> MGSSHHHHHHSSGLVPRGSHMTTTISADQ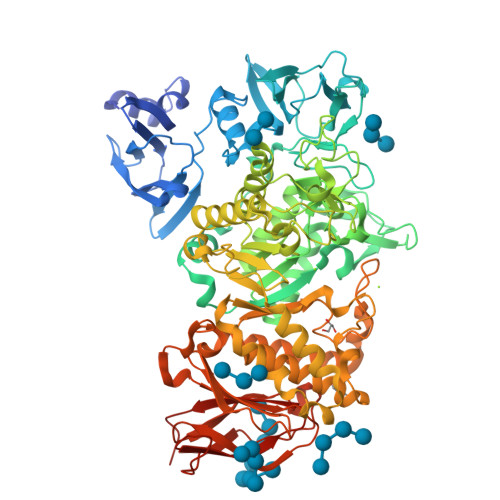VNQIIYNLHHDPFEILGCHLLEEGKNTKKWVVRAYLPKAEAAWVIRPTERKEDPMNSVHHPNFFECIIETPELNHYQLKVKEGEHEKVIYDPYAFSSPYLTDEDIYLFSEGNHHRIYEKLGAHVGEINGVKGVYFAVWAPNARNVSVIGDFNNWDGREHQMRKRNYTIWELFVPEIGSGTVYKYEIKNSEGHIYEKSDPYGFYREVRPNTASIVVDIDNIYQWHDEEWLEKRRNSDPLKQPVSVYEVHLGSWLHGSSAEKMPLLNGEADPVIVSEWNPGARFLSYYELAEKLIPYVKDMGYTHIELLPIAEHPFDGSWGYQVTGFYSPTSRFGRPEDFMYFVDKCHENGIGVILDWVPGHFPKDSHGLAYFDGTHLYEHADPRIGEHKEWGTLVFNYGRHEVRNFLVANVLFWFDKYHVDGIRVDAVASMLYRNYLRKEGEWIANEYGGDEHIEAVSFIREVNTLLFEYFPGILSIAEESTEWEKVSRPVAAGGLGFNLKWDMGWMHDMLDYFNIDPYFRQYHQNNVTFSMLYYYNENFMLALSHDEIVHGKSNMLGKMPGDEWQKYANVRALFTYMYTHPGKKTMFMSMEFGQWSEWNVWGDLEWHLLQYEPHQQLKQFFTDLNALYQQEPALYTHDFEYHGFEWIDCNDNTHSVVSFLRRSDDPNDSLVVVCNFTPQPHSHYRIGVPEAGYYVELFNSDAKQYGGSNMGNLGGKWADEWSFHNKPYSLDLCLPPLAVLILKLDPTKVPEGTTIKEIAADEEE> GAMDPMIIRGIRGARINNEIFNLGLKFQILNADVVATKKHVLHAINQAKTKKPIAKSFWMEILVRASG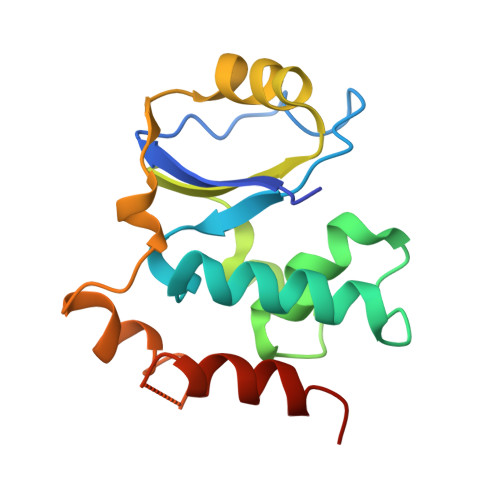QRQIHEAIKIIGAKDGNVCLICEDEETFRKIYELIGGEIDDSVLEINEDKERLIREIFKIRGFGNVVERVLEKIALIELKKE>GTILWDG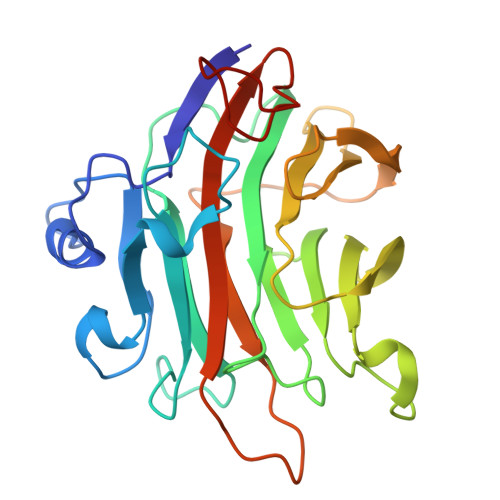RFNDMTSSADLNKWSWGNQVGPYQYYIHGSSPVSAYVNLSPDYKNPADTGSRQGAKITLDNTAYWNGQNMRRTELIPQTTAAINQGKVYYHFSLMRKDINAPATTREHQIAFFESHFTELKSGWLSGAPGISDTLLRWCVGGQTQWSVEWAADVWHNVAYEIDFAAGTVGFWHSTGSDPLTRKVAPVKTSTSSNGADWHVGVLELPRSGYPDSNEDFYWSGVYIESGSLTTSVAGPGQPIPGDGG[4x]(3E)-5-fluoro-1-[(6-fluoro-4H-1,3-benzodioxin-8-yl)methyl]-1H-indole-2,3-dione 3-oxime | C17 H12 F2 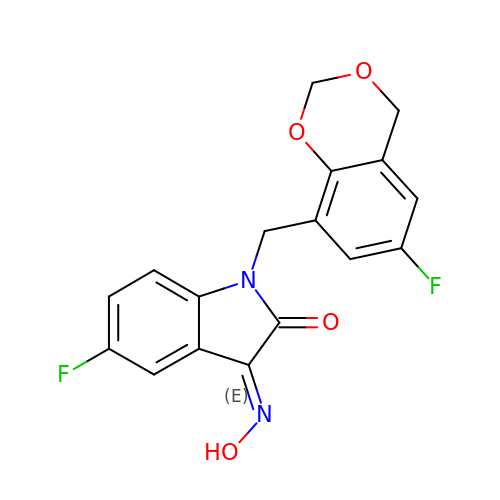N2 O4 | DXIHOIDYHQSQKJ-HMMYKYKNSA-N> ART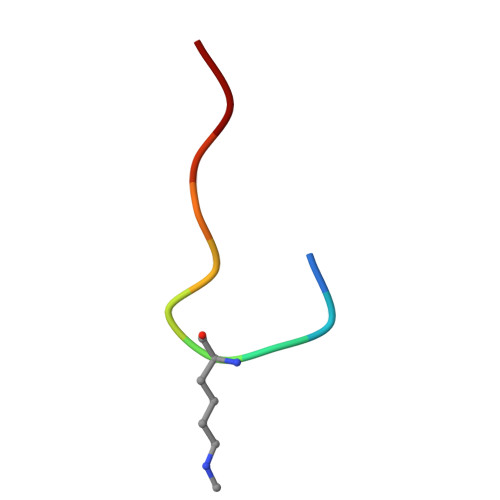KQTARKY The PWWP domain comprises 100–130 amine acids and is often present in chromatin-associated proteins. Our structures revealed that the overall fold of the PWWP domain consists of three motifs: a canonical β-barrel core, an insertion motif between the second and third β-strands and a C-terminal α-helix bundle. The canonical β-barrel core harbors an aromatic cage constructed by three aromatic residues, which is a signature feature of the Tudor domain “Royal family”. Taken together, similar to other members in the ‘Royal family’, PWWP domain also exhibits methyllysine histone binding ability.

In order to explore the functional roles of the PWWP domains, we determined the crystal structures of the PWWP domains from 7 different human proteins, namely, BRPF1 (bromodomain and PHD finger-containing protein 1), BRPF2, BRPF3, MUM1 (melanoma associated antigen (mutated) 1), DNMT3A, DNMT3B and HDGF2 (Hepatoma-derived growth factor 2). By fluorescence polarization assay, we found that the PWWP domains in BRPF1, BRPF2, HDGF2, MUM1 and the N-terminal PWWP domains of WHSC1 and WHSC1L1 show weak binding affinity to histones with H3K36, K3K79 or H4K20 methylation.

>EPRSFEVGMLVWHKHKKYPFWPAVVKSVRQRDKKASVLYIEGHMNPKMKGFTVSLKSLKHFDCKEKQTLLNQAREDFNQDIGWCVSLITDYRVRLGCGSFAGSFLEYYAADISYPVRKSIQQDVLGTKLPQLSK[4x]N-(5-phenylpentyl)adenosine | C21 H27 N5 O4 | 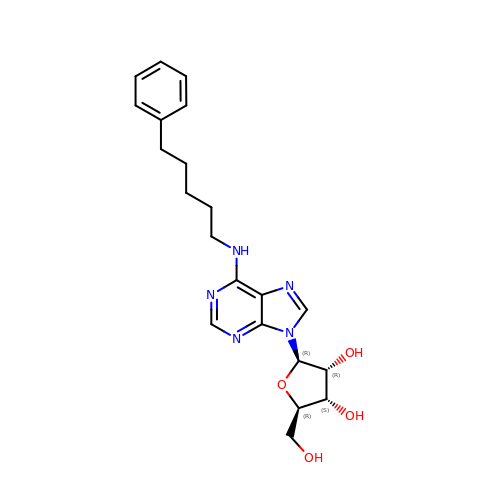OWDHJJGXMJRIBB-QTQZEZTPSA-N> ELTQSRVQKIWVPNSPTVIVMVGLPARGKTYISKKLTRYLNWIGVPTKVFNVGEYRREAVKQYSSYNFFRPDNEEAMKVRKQCALAALRDVKSYLAKEGGQIAVFDATNTTRERRHMILHFAKENDFKAFFIESVCDDPTVVASNIMEVKISSPDYKDCNSAEAMDDFMKRISCYEASYQPLDPDKCDRDLSLIKVIDVGRRFLVNRVQDHIQSRIVYYLMNIHVQPRTIYLCRHGENEHNLQGRIGGDSGLSSRGKKFASALSKFVEEQNLKDLRVWTSQLKSTIQTAEALRLPYEQWKALNEIDAGVCEELTYEEIRDTYPEEYALREQDKYYYRYPTGESYQDLVQRLEPVIMELERQENVLVICHQAVLRCLLAYFLDKSAEEMPYLKCPLHTVLKLTPVAYGCRVES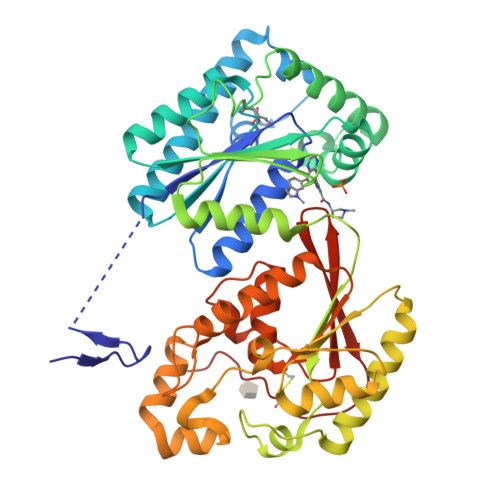IYLNVESVCTHRERSE ETHYL (4R)-4-{[N-(TERT-BUTOXYCARBONYL)-L-PHENYLALANYL]AMINO}-5-[(3S)-2-OXOPYRROLIDIN-3-YL]PENTANOATE | C25 H37 N3 O6 | 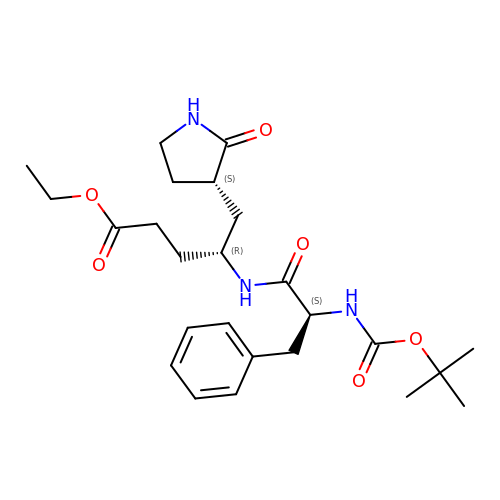CUCJJUOQGSQGLL-ZCNNSNEGSA-N> GTXTSDY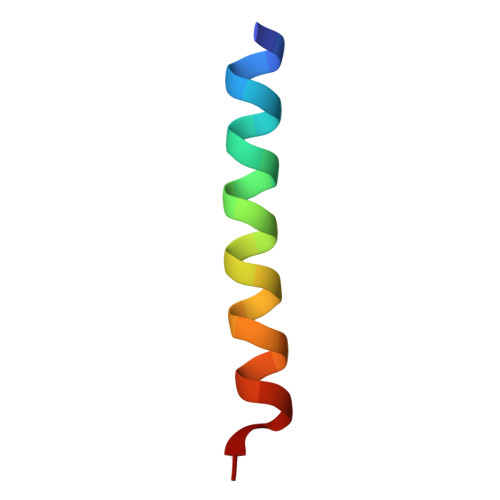SKYLDSRRAQDXVQWLMNT> GSATVTVTFTITELCLRTGVSEEELTEIVGLGMIEPHQPQADTWLFDDSAVTIVHRAVRLRNELELDWPGIAVALTLLDENARLTRENRLL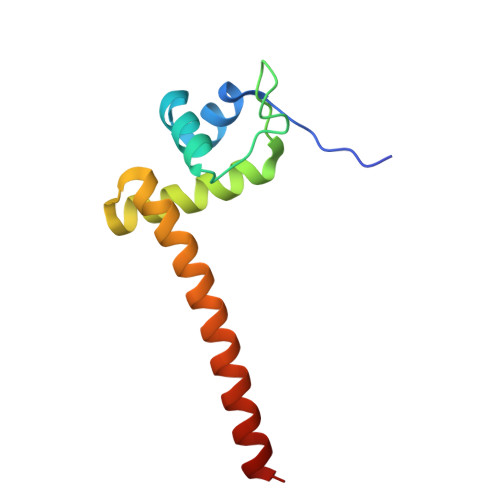QQRLARFLAHG> GAASEEVEQTPLQEALNQLMRQLQRKDPSAFFSFPVTDFIAPGYSMIIKHPMDFSTMKEKIKNNDYQSIEELKDNFKLMCTNAMIYNKPETIYYKAAKKLLHSGMKI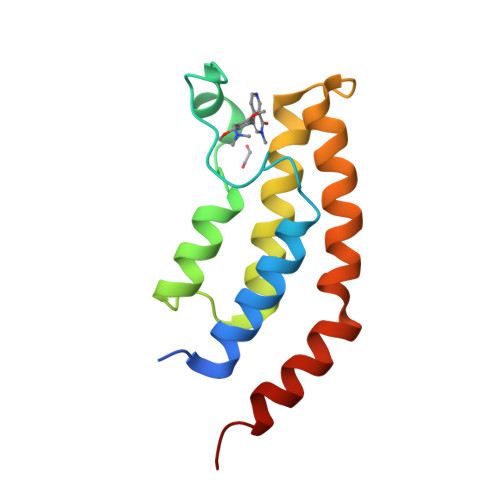LSQERIQSLKQSIDFMADL> ETVPD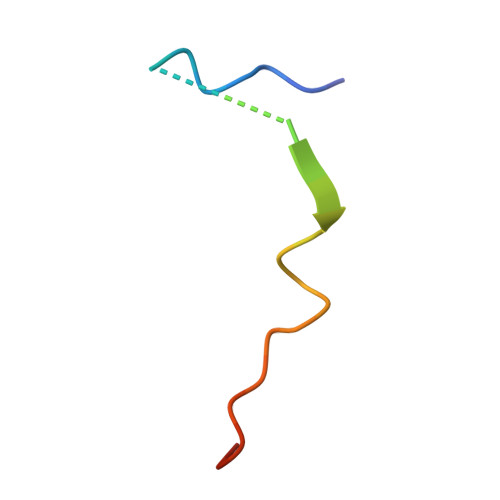SQISGFDSPLIPTSVGSYFRDDDD> LDHLHAAEAAYQIESIIKTATDTVKSEINAELGVVPSLNAVETGATSNTEPEEAIQTRTVINQHGVSETLVENFLSRAALVSKRSFEYKDHTSSTARADKNFFKWTINTRSFVQLRRKLELFTYLRFDAEITILTTVAVNGSGNNTYVGLPDLTLQAMFVPTGALTPEKQDSFHWQSGSNASVFFKISDPPARITIPFMCINSAYSVFYDGFAGFEKNGLYGINPADTIGNLCVRIVNEHQPVGFTVTVRVYMKPKHIKAWAPRPPRTLPYMSIANANYKGKERAPNALSAIIGNRDSVKTMPHNIVNT;> GVPTYLLPGSGQFLTTDDHSSAPALPCFNPTPEMHIPGQVRNMLEVVQVESMMEINNTESAVGMERLKVDISAL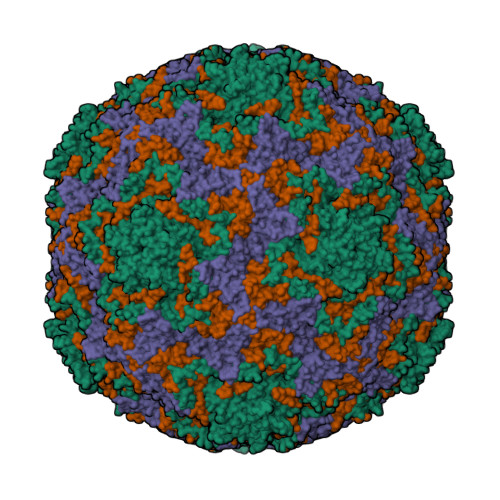TDVDQLLFNIPLDIQLDGPLRNTLVGNISRYYTHWSGSLEMTFMFCGSFMAAGKLILCYTPPGGSCPTTRETAMLGTHIVWDFGLQSSVTLIIPWISGSHYRMFNNDAKSTNANVGYVTCFMQTNLIVPSESSDTCSLIGFIAAKDDFSLRLMRDSPDIGQLDHLHAAEAAYQ;> SPSAEACGYSDRVLQLKLGNSAIVTQEAANYCCAYGEWPNYLPDHEAVAIDKPTQPETATDRFYTLKSVKWETGSTGWWWKLPDALNNIGMFGQNVQHHYLYRSGFLIHVQCNATKFHQGALLVVAIPEHQRGAHNTNTSPGFDDIMKGEEGGTFNHPYVLDDGTSLACATIFPHQWINLRTNNSATIVLPWMNAAPMDFPLRHNQWTLAIIPVVPLGTRTTSSMVPITVSIAPMCCEFNGLRHAITQ;> MGAQVTRQQTGTHENANIATNGSHITYNQINFYKDSYAASASKQDFSQDPSKFTEPVVEGLKAGAPVLK> MTTYGSSVPEQQITAYLSRIQRGGYIQPFGCMIAVDESSFRIIGYSENAREMLGIMPQSVPTLEKPEILAMGTDVRSLFTSSSSILLERAFVAREITLLNPVWIHSKNTGKPFYAILHRIDVGVVIDLEPARTEDPALSIAGAVQSQKLAVRAISQLQALPGGDIKLLCDTVVESVRDLTGYDRVMVYKFHEDEHGEVVAESKRDDLEPYIGLHYPATDIPQASRFLFKQNRVRMIVDCNATPVLVVQDDRLTQSMCLVGSTLRAPHGCHSQYMANMGSIASLAMAVIINGNEDDGSNVASGRSSMRLWGLVVCHHTSSRCIPFPLRYACEFLMQAFGLQLNMELQLALQMSEKRVLRTQTLLCDMLLRDSPAGIVTQSPSIMDLVKCDGAAFLYHGKYYPLGVAPSEVQIKDVVEWLLANHADSTGLSTDSLGDAGYPGAAALGDAVCGMA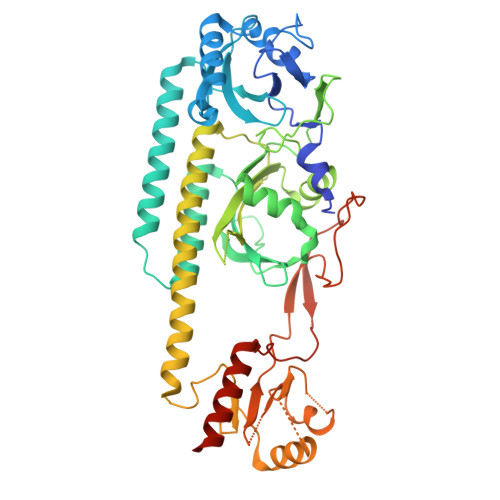VAYITKRDFLFWFRSHTAKEIKWGGAKHHPEDKDDGQRMHPRSSFQAFLEVVKSRSQPWETAEMDAIHSLQLILRDSFKESEAASLHHHHHH>[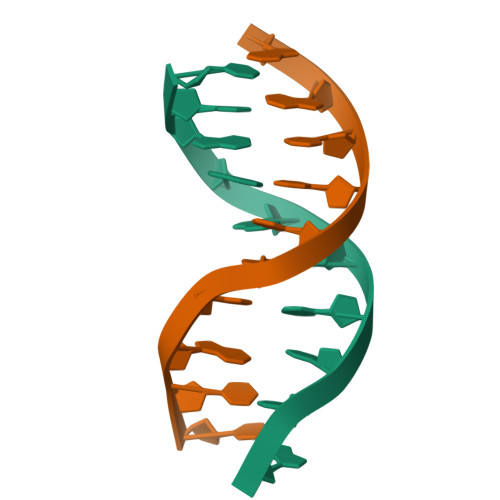2x]CCGAGCTCGG4-nitro-2-phosphonobenzoic acid | C7 H6 N O7 P | 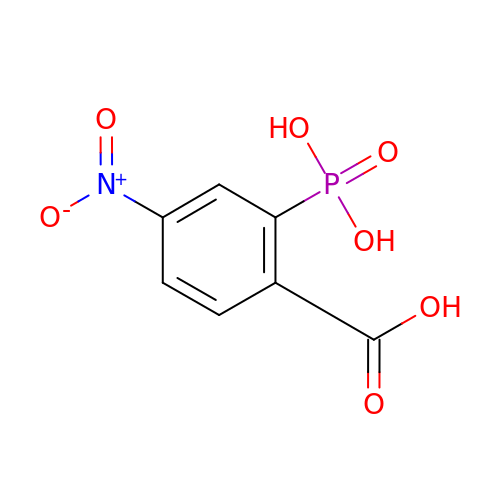PFWUFGANONPVGT-UHFFFAOYSA-N>[10x]MEKFRAVLDLHVKHHSALGYGLVTLLTAGGERIFSAVAFQCPCSAAWNLPYGLVFLLVPALALFLLGYVLSARTWRLLTGCCSSARASCGSALRGSLVCTQISAAAALAPLTWVAVALLGGAFYECAATGSAAFAQRLCLGRNRSCAAELPLVPCNQAKASDVQDLLKDLKAQSQVLGWILIAVVIIILLIFTSVTRCLSPVSFLQLKFWKIYLEQEQQILKSKATEHATELAKENIKCFFEGSHPK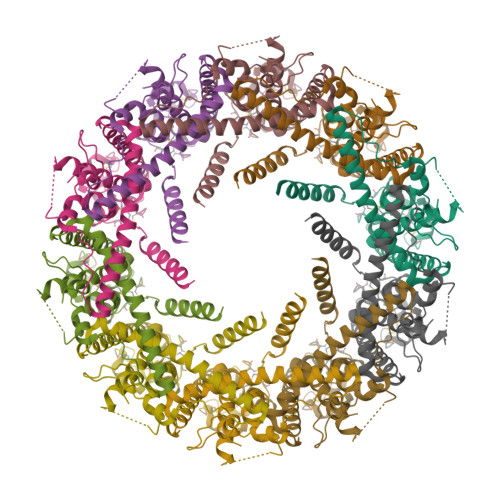EYNTPSMKEWQQISSLYTFNPKGQYYSMLHKYVNRKEKTHSIRSTEGDTVIPVLGFVDSSGINSTPEL>GSMKKERVITEFWDGKIIMVSPDDPKYALKKAEEVRELVDSELGFQQVSLRCPSQTRTYMFVSNEKKIVGCLIAEPIREAYRVLAEPPSLHSLHGEPLERHRAWRCSTEPEPAICGISRIWVFALMRRKAIASRMVDAVR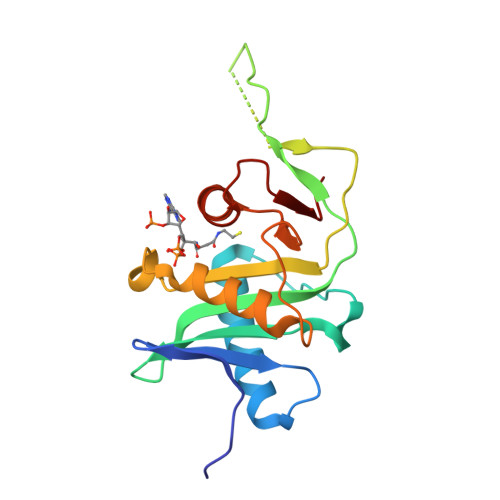SSFMYGSVLTTEEIAFSDPTPDGKLFASTYCKVPDFLVYNFVS[2x]>[16x]MGRDAQRMNILAGRIIAETVRSTLGPKGMDKMLVDDLGDVVVTNDGVTILREMSVEHPAAKMLIEVAKTQEKEVGDGTTTAVVVAGELLRKAEELLDQNVHPTIVVKGYQAAAQKAQELLKTIACEVGAQDKEILTKIAMTSITGKGAEKAKEKLAEIIVEAVSAVVDDEGKVDKDLIKIEKKSGASIDDTELIKGVLVDKERVSAQMPKKVTDAKIALLNCAIEIKETETDAEIRITDPAKLMEFIEQEEKMLKDMVAEIKASG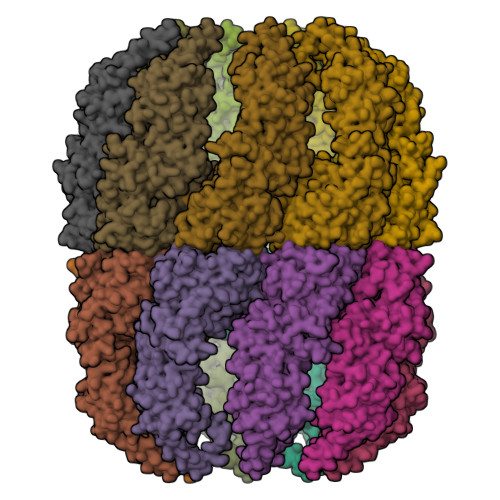ANVLFCQKGIDDLAQHYLAKEGIVAARRVKKSDMEKLAKATGANVITNIKDLSAQDLGDAGLVEERKISGDSMIFVEECKHPKAVTMLIRGTTEHVIEEVARAVDDAVGVVGCTIEDGRIVSGGGSTEVELSMKLREYAEGISGREQLAVRAFADALEVIPRTLAENAGLDAIEILVKVRAAHASNGNKCAGLNVFTGAVEDMCENGVVEPLRVKTQAIQSAAESTEMLLRIDDVIAAEKLR>[2x]MGSSHHHHHHSSGRENLYFQGMNIMPISESQLSDWLALRCLLWPDHEDVHLQEMRQLITQAHRLQLLAYTDTQQAIAML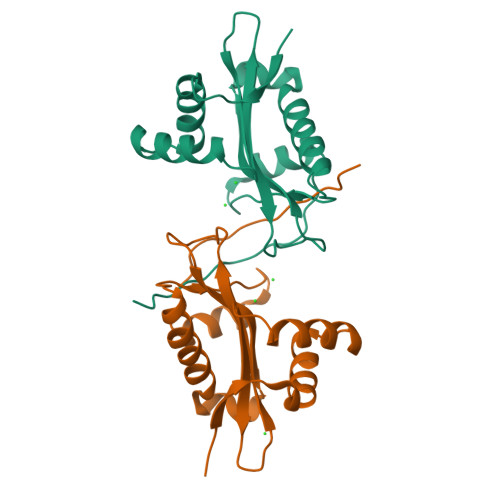EASIRYEYVNGTQTSPVAFLEGIFVLPEYRRSGIATGLVQQVEIWAKQFACTEFASDAALDNQISHAMHQALGFHETERVVYFKKNIG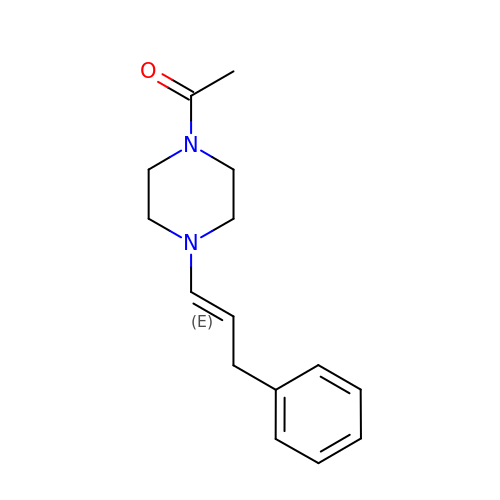1-{4-[(1E)-3-phenylprop-1-en-1-yl]piperazin-1-yl}ethan-1-one | C15 H20 N2 O | ZITAIQWIBNEJAO-WEVVVXLNSA-N> GPLGSMAAAPPLRDRLSFLHRLPILLKGTSDDDVPCPGYLFEEIAKISHESPGSSQCLLEYLLSRLHSSSGHGKLKVLKILLYLCSHGSSFFLLILKRNSAFIQEAAAFAGPPDPLHGNSLYQKVRAAAQDLGSTLFSDTVLPLA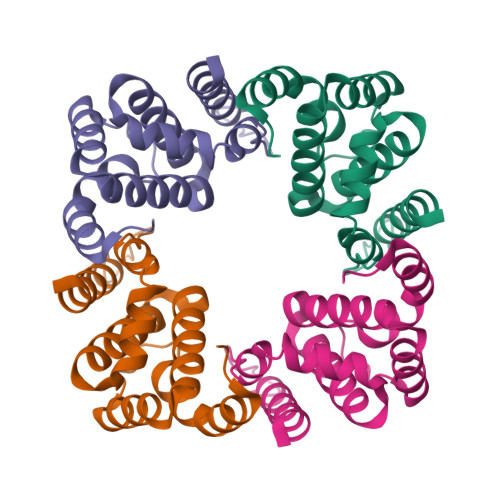PSQPLGTPPATGM> MSKIAKTAIISPKAEINKGVEIGEFCVIGDGVKLDEGVKLHNNVTLQGHTFVGKNTEIFPFAVLGTQPQDLKYKGEYSELIIGEDNLIREFCMINP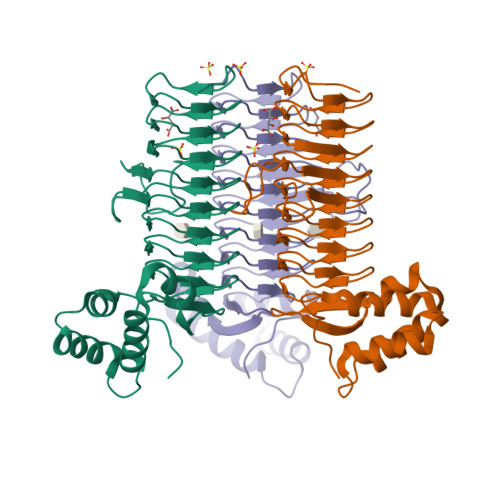GTEGGIKKTLIGDKNLLMAYVHVAHDCVIGSHCILANGVTLAGHIEIGDYVNIGGLTAIHQFVRIAKGCMIAGKSALGKDVPPYCTVEGNRAFIRGLNRHRMRQLLESKDIDFIYALYKRLFRPIPSLRESAKLELEEHANNPFVKEICSFILESSRGVAYKSSEYSSEEKQEE>TPDCVTGKVEYTKYNDDDTF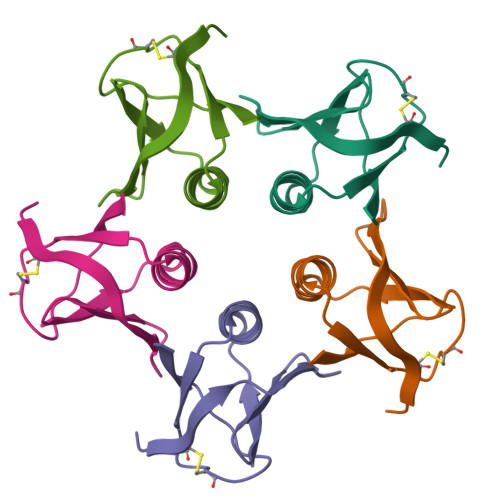TVKVGDKELFTNRWNLQSLLLSAQITGMTVTIKTNACHNGGTFSEVIFR[5x]>[4x]MASMTGGQQMGRGSMPLLAQEAITRAKTMMKPFILRRRKDQVLKHLPPKHTHIQYCELNAIQKKIYDKEIQIVLEHKRMIKDGELPKDAKEKSKLQSSSSKNLIMALRKASLHPLLFRNIYNDKIITKMSDAILDEPAYAENGNKEYIKEDMSYMTDFELHKLCCNFPNTLSKYQLHNDEWMQSGKIDALKKLLKTIIVDKQEKVLIFSLFTQVLDILEMVLSTLDYKF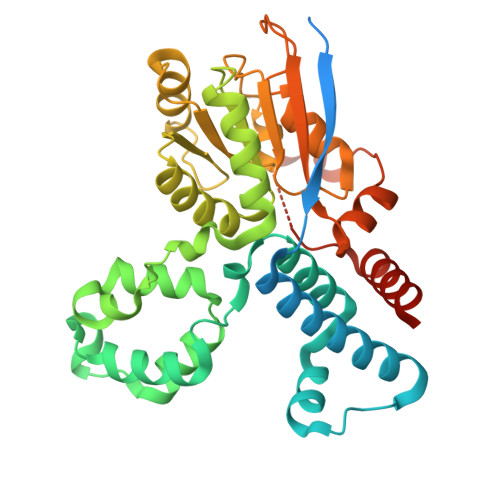LRLDGSTQVNDRQLLIDKFYEDKDIPIFILSTKAGGFGINLVCANNVIIFDQSFNPHDDRQAADRAHRVGQTKEVNITTLITKDSIEEKIHQLAKNKLALDSYISEDKKSQDVLESKVSDMLEDIIYDELEHHHHHH>[2x]ALPTIHVVTPTY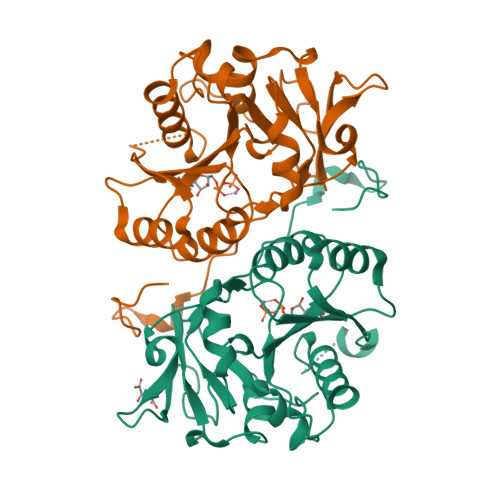SRPVQKAELTRMANTLLHVPNLHWLVVEDAPRRTPLTARLLRDTGLNYTHLHVETPRNYKLRGDARDPRIPRGTMQRNLALRWLRETFPRNSSQPGVVYFADDDNTYSLELFEEMRSTRRVSVWPVAFVGGLRYEAPRVNGAGKVVRWKTVFDPHRPFAIDMAGFAVNLRLILQRSQAYFKLRGVKGGYQESSLLRELVTLNDLEPKAANCTKILVWHTRTEKPVLVNEGKKGFTDPSVEI(11Z,13Z)-hexadeca-11,13-dienal | C16 H28 O | 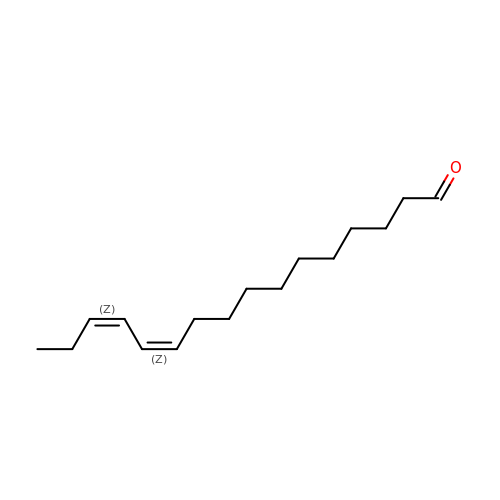ZTJGMVSDMQAJPE-OUPQRBNQSA-N>[2x]GSFKLTILHTNDVHARLEQTSRDSGKCSGEDCYGGVARRATKIRQIRASHRNVLLLDAGDQYQGTIWFNYFKGREVVHFMNSLRYDAMALGNHEFDNGLNGLLDPLLKNVKFPILSANIRPKGPIASKISGYILPYKIINVGSEKVGIIGYTTKETPVLSNPGPYLEFRDEVEELQKHADKLTTLGVNKIIALGHSGFMEDCRIAQKVKGVDVVVGGHTNTFLYTGSP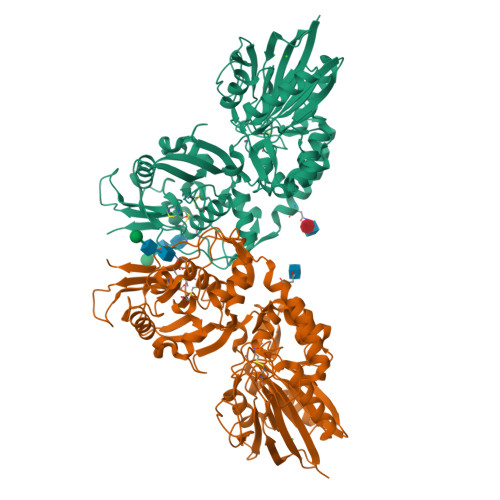PSNEVAAGNYPFMQLSDDGRQVPVVQAYAFGKYLGYLNVIFDDKGKVIKASGNPILLNKSIQEDPAVKAEISRMKVQLQNYSSQEIGRTIVYLNGTTHACRFHECNLGNLICDAVVYNNLRHPDDNEWNHVSMCIVNGGGIRSPIDEQANNGIITLEELTAVLPFGGTFDLLQIKGSTLRQAFEHSVHRHGQGTGELLQVSGIKVVYDLSQKPGKRVVSLNVLCTECRVPTYVPLEMEKTYKVLLPSFLAAGGDGYYMLKGDSSNHSSGDLDISIVGNYIKRMGKVFPAMEGRMVFSAGTLF>[6x]NLYFQGAMGSTCGAWEMKERLGTGGFGNVIRWHNQETGEQIAIKQCRQELSPRNRERWCLEIQIMRRLTHPNVVAARDVPEGMQNLAPNDLPLLAMEYCQGGDLRKYLNQFENCCGLREGAILTLLSDIASALRYLHENRIIHRDLKPENIVLQQGEQRLIHKIIDLGYAKELDQGELCTEFVGTLQYLAPELLEQQKYTVTVDYWSFGTLAFECITGFRPFLPNWQPVQWH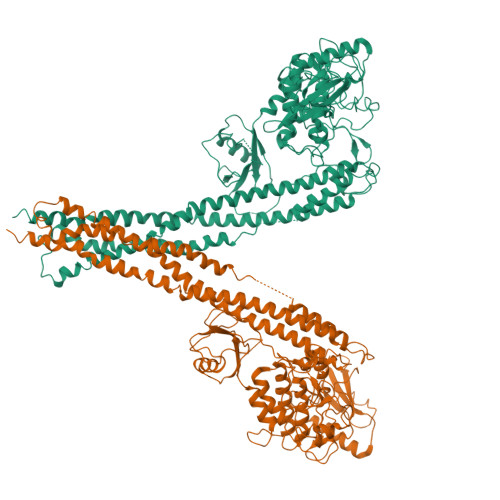SKVRQKSEVDIVVSEDLNGTVKFSSSLPYPNNLNSVLAERLEKWLQLMLMWHPRQRGTDPTYGPNGCFKALDDILNLKLVHILNMVTGTIHTYPVTEDESLQSLKARIQQDTGIPEEDQELLQEAGLALIPDKPATQCISDGKLNEGHTLDMDLVFLFDNSKITYETQISPRPQPESVSCILQEPKRNLAFFQLRKVWGQVWHSIQTLKEDCNRLQQGQRAAMMNLLRNNSCLSKMKNSMASMSQQLKAKLDFFKTSIQIDLEKYSEQTEFGITSDKLLLAWREMEQAVELCGRENEVKLLVERMMALQTDIVDLQRSPMGRKQGGTLDDLEEQARELYRRLREKPRDQRTEGDSQEMVRLLLQAIQSFEKKVRVIYTQLSKTVVCKQKALELLPKVEEVVSLMNEDEKTVVRLQEKRQKELWNLLKIACSKVRGPV> SLVSIDLPIEGRLARYDLTGRPVPFNSRDAKAFSRVAFAAAHVVADPLADNDPWLAPAIDWERTLAFRHRLWDLGLGVAESMDTAQRGMGLGWPEARELIRRSLAEARGRPDALIACGAGTDHLAPGPDVSIDDILAAYESQIEAIEAEGGRIILMASRALAAAAKGPEDYIRVYDRVLSQVKEPVIIHWLGEMFDPALEGYWGNADHMAAMKTCLDVLEAHAAKVDGIKISLLSKEKEIVMRRQLPKG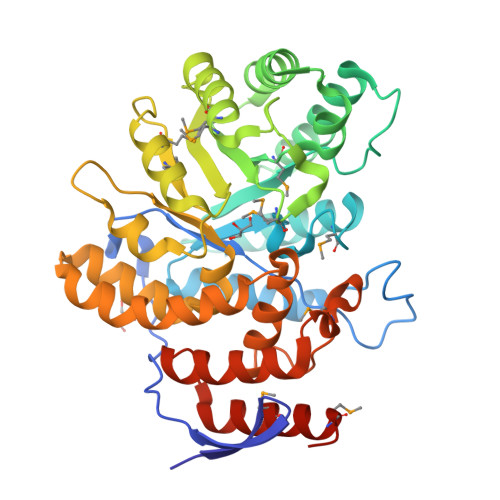VRMYTGDDFNYAELIAGDEEGHSDALLGIFDAIAPVASAALEALGSGRNGEFFELLEPTVPLSRHIFKAPTRFYKTGVVFLAYLNGLQDHFVMIGGQQSARSLVHLAELFRLADKAGALADPELATARMRRVLAMHGVEEGHHHHHH> LVPRGSEDKWRNAFDHMLMEEFEEKMDQIEHGLLMLSEQYKELEKTKSKELKEQILRELTIAENYLRGALKFMQQEAKRTDLNMFERYNFETAVSTIEILVKDLAELAKKVKAVKSD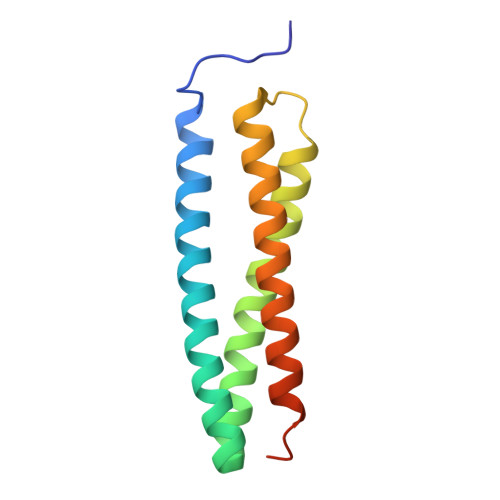DGSHHHHH>[3x]SMLKEASNESGTWARACDTCRSAACTVYCEADSAYLCTTCDARVHAANRV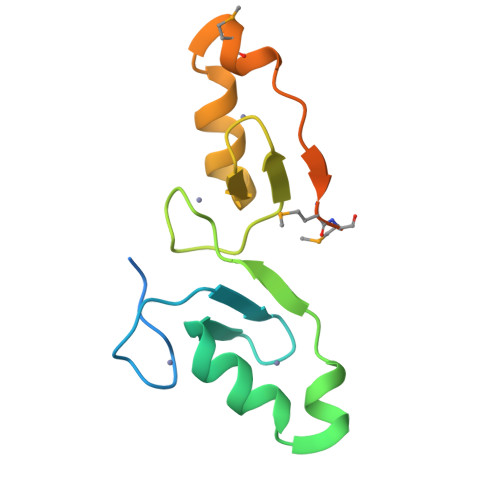ASRHERVRVCQSCESAPAAFLCKADAASLCTACDAEIHSANPMARRHQRVPMMPLSANSCSSMAPSETDAD>GGSGNEPTQEKHFMVYYRAWRDKTMQGVNTTLPDENWLTMHDIPYGIDIVNVFSYVPKGQEALAQPFYDTLKNEYAPALHARGVRLVRGIDYSELLKVPYAGTTPTEAEFDAYAKELLTKFVDDLGIDGLDIDMETRPSEKDIVLSNGVIRALSKYIGPKSGTDRPFLYDTNAEYLPPLQDVSDCFDFLAYQQYGSDDKRTQRALNNLSPVLNGERFVPGLTFPEEQDRNRWYDTKEPYMESNMYKVARYSYENNLGGMFLYALDRDGRTYNEDDLNQIKPSNLLWTKTAIAESKGVSLAEMKAAAQHYLKRISYANTDLEAQNKAAETVTQATTLYDVNKAILGGDYGQGLSNTYDAELEKGLLAIDLTTLYRALDQAVAAIEKAESYTPETIQALQTTKESVATELAGKTYTAAQVTTWQTEVQTALDNLKEK[2x]

Here we focus on EndoE, a multi-modular glycoside hydrolase secreted by Enterococcus faecalis, one of the leading causes of healthcare-associated infections. We provide X-ray crystal structures of EndoE, which show an architecture composed of four domains, including GH18 and GH20 glycoside hydrolases connected by two consecutive three α-helical bundles. We determine that the GH20 domain is an exo-β-1,2-N-acetylglucosaminidase, whereas the GH18 domain is an endo-β-1,4-N-acetylglucosaminidase that exclusively processes the central core of complex-type or high-mannose-type N-glycans. Both glycoside hydrolase domains act in a concerted manner to process diverse N-glycans on glycoproteins, including therapeutic IgG antibodies.

EndoE-GH18L-Man5 crystallized in the C 1 2 1 space group with two molecules in the asymmetric unit and diffracted to a maximum resolution of 2.6 Å. The structural comparison of EndoE-GH18L and the product bound EndoE-GH18L-Man5 revealed that the protein structure is mostly preserved upon glycan binding and that there are no substantial conformational changes (r.m.s.d. of 0.58 Å for 416 residues). The Man5 product could be modelled unambiguously in the electron density map, located at the center of the (β/α)8-barrel and surrounded by the loops 1 to 8. The GlcNAc (-1) residue adopts a chair conformation (4C1) in which O1 makes hydrogen bonds with the side chains of E186 and Q243, and O3 establishes an intramolecular hydrogen bond with the cyclic oxygen atom in the Man (-2) ring. The N2 atom of the acetamide group interacts through hydrogen bonds with the side chains of D184 and E186, whereas the O7 atom makes a hydrogen bond with the side chain of Y245. This conformation likely corresponds to a stage of the catalytic cycle of the enzyme shortly before the release of the glycan product. The crystal structure of the EndoE-GH18L-Man5 complex reveals that the Man5 glycan is accommodated in a groove that forms a narrow space for the α(1,3) antenna. Specifically, loop 1 of the GH18 domain clearly restricts the access of additional Man residues with respect to Man (-6). In that sense, our crystal structure of the EndoE-GH18L-Man5 complex unveils the molecular mechanism of HM-type N-glycan substrate recognition and specificity of EndoE. Supporting this notion, the crystal structure of the EndoE-GH18L-Man5 complex and docking calculations of EndoE-GH18L with Man6, Man7, and Man9 show that Man6 can bind to the active site of the GH18 domain because the additional mannose (Man (-7)) of the α(1,3) antenna can interact with loop 1 of the enzyme.> MALDRPDRSGAVRVSAPARLSFTLISLDGSSLRRNGIAAMAVDRPGLTAEVREAADGIVAVTGTAEETARELAAALEALRKLWDGPAARVDVLEALPQHSGFGSKTSTLLAVGHAYGRLCGVEPDLRELARTLGRGRVSGASTGLSAYGGFLVDGGHVNPPDFAE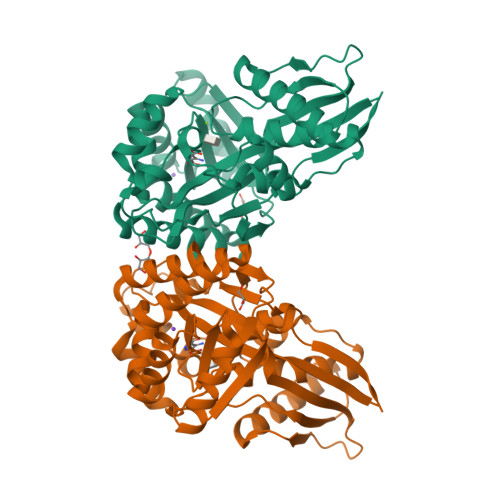APQKYLRPSRFAQQVAPPKPVVRLDFPDWPVLVLLTHGRHLGGQEELEWFHSVAPIPAEESWRTSHLVFMGLAPAVLEQDFDAFCAAVNEITFTGHFKQAQIAFQGDAVADVLEAGRAAPSVDAIALSVTGPACFAFTKRPEDAERWAWELKNRGLIRDFWFTRANNQGLATTVVS Hence, this loss of critical proteins has the potential to compromise ER proteostasis and generate cellular stress. This challenge to normal metabolism is overcome by the activity of the cytosolic coatomer protein I (COPI) polymer, whose repeating unit is the coatomer, a 560 kDa complex of seven distinct gene products (α-, β-, β′-, γ-, δ-, ε-, and ζ-COPI)25–31. Overall, the coatomer functions to retrieve the escaped “client” proteins, such as type I membrane proteins, from cis-Golgi back to ER by retrograde trafficking. In particular, the S protein – a type I membrane protein – is delivered to the ERGIC from both the ER (by anterograde trafficking) and the Golgi (by retrograde trafficking)3,10–12. Here we utilize recombinant SARS-CoV-2 S proteins and tail peptides, including constructs with enhanced mimicry of the coatomer binding motif (clientized S protein), to elucidate the atomic structure of the S-coatomer interface.

To gain insight into the role of the basic cluster in stabilizing S-coatomer interactions, we generated alanine mutants of αWD40 Arg13, Lys15, and Arg300, which are equivalent to the β‘WD40 basic cluster residues Arg15, Lys17, and Arg272, respectively. Biolayer interferometry (BLI) assays showed that Arg13Ala weakened αWD40 binding to both wild-type and clientized Thr1273Glu S heptapeptides, although the affinity for the clientized S heptapeptide was still 2.8-fold higher. A 1.9 Å resolution crystal structure of this αWD40 Arg13Ala mutant showed a binding site architecture comparable to that in wild-type αWD40, attributing affinity weakening to the alanine mutation. F Superposition of wild-type (white) and Arg13Ala mutant (yellow) crystal structures shows minimal perturbation near the mutation site. In contrast, Arg13 and Lys15 residues in αWD40 provide the basis for basal binding to both wild-type and clientized S molecules.

>[3x]MEMLTKFESRSSAAKGVAFHPTQPWILTSLHNGRIQLWDYRMGTLLDRFDGHDGPVRGIAFHPTQPLFVSGGDDYKVNVWNYKSRKLLFSLCGHMDYVRVCTFHHEYPWILSCSDDQTIRIWNWQSRNCIAILTGHSHYVMCAAFHPSEDLIVSASLDQTVRVWDISGLRMKNAAPVSMSKEDQKAQAHNSKSNDKKGSTDAIVKFVLEGHDRGVNWCAFHPTLPLILSAGDDRLVKLWRMTASKAWEVDTCRGHFNNVSCCLFHPHQELILSASEDKTIRVWDLNRRTAVQTFRRDNDRFWFITVHPKLNLFAAAHDSGVMVFKLESAWSHPQFEK>[4x]MPRDNMASLIQRIARQACLTFRGSSTGSEGPAPGFPENLSLLKSLLTQVRAEDLNIAPRKALPQPLPRNLPPVTYMHIYETEGFSLGVFLLKSGTCIPLHDHPGMHGMLKVLYGTVRISCMDKLDTGAGHRRPPPEQQFEPPLQPLE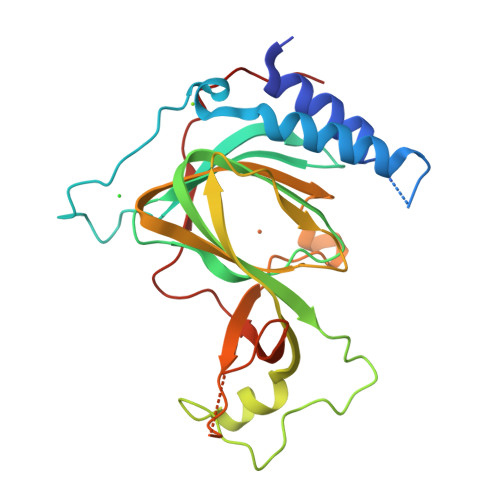REAVRPGVLRSRAEYTEASGPCVLTPHRDNLHQIDAVDGPAAFLDILAPPYDPEDGRDCHYYRVVEPIRPKEASGSACDLPREVWLLETPQADDFWCEGEPYPGPKVLP>[2x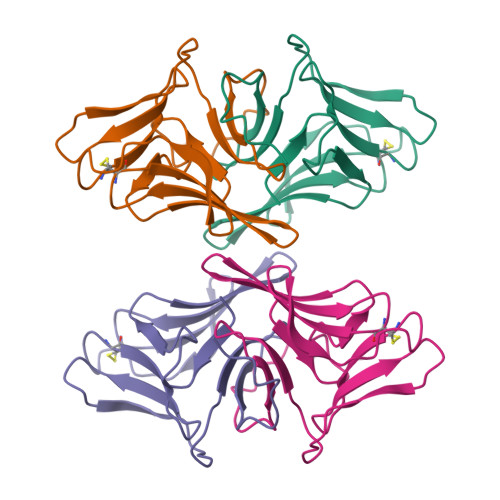]NNIIFSKQPDDNHPQILHATESLEILFGTHVYRFIMQTDCNLVLYDNNNPIWATNTGGLGNGCRAVLQPDGVLVVITNENVTVWQSPVAGKAGHYVLVLQPDRNVVIYGDALWATQTVR> GPLGSEILRHSMDPATFTFNFNNEPWVRGRHETYLCYEVERMHNDTWVKLAQRRGFLANQAKHKHGFLEGRHAALCFLDV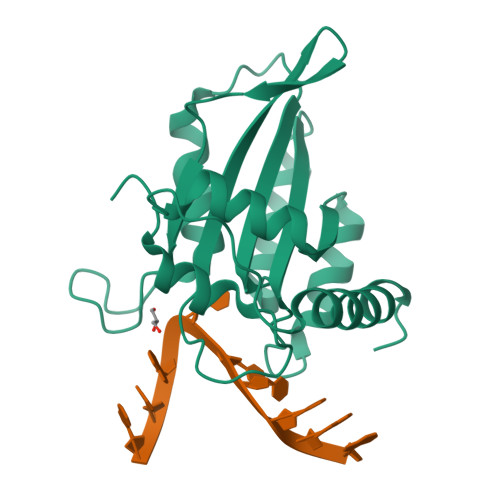IPFWKLDLDQDYRVTCFTSWSPCFSCAQEMAKFISKNKHVSLCIKTARIYDDKGRAAEGLRTLAEAGAKISIMTYSEFKHCWDTFVDHQGAPFQPWDGLDEHSQDLSGRLRAILQNQEN> MTTQEFLSKNKTIESELLDLLIKPNTDDSILTRNKQAIADRDLFDIEWEPGQSLNKLATEYLGDSFAWQIIADANGIDPTKEID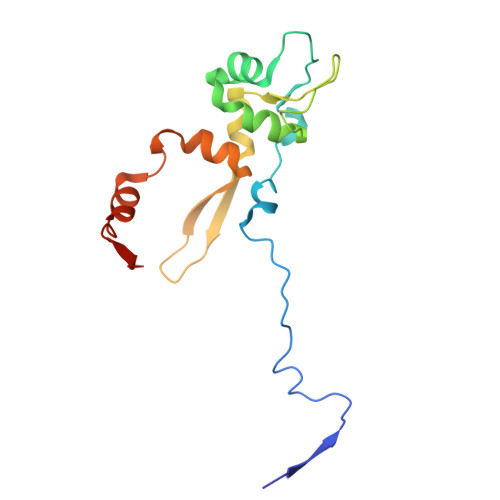IGAGLKVPDQKALENSIKKFIVNSPTGKQLISDAKQSILNLIGVGDSNTEFSKTLKDCIGKVVNFSFDNTQ(4S)-4-(3-HYDROXYPHENYL)-7,7-DIMETHYL-2-THIOXO-2,3,4,6,7,8-HEXAHYDROQUINAZOLIN-5(1H)-ONE | C16 H18 N2 O2 S | 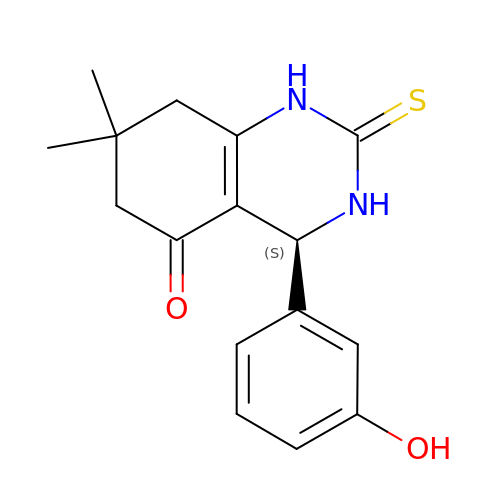RUOOPLOUUAYNPY-AWEZNQCLSA-N>PMVTAATSLRRALENPDSFIVAPGVYDGL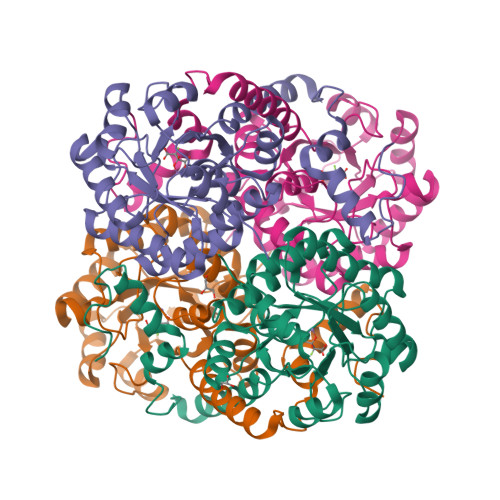SARVALSAGFDALYMTGAGTAASVHGQADLGICTLNDMRANAEMISNISPSTPVIADADTGYGGPIMVARTTEQYSRSGVAAFHIEDQVQTKRCGHLAGKILVDTDTYVTRIRAAVQARQRIGSDIVVIARTDSLQTHGYEESVARLRAARDAGADVGFLEGITSREMARQVIQDLAGWPLLLNMVEHGATPSISAAEAKEMGFRIIIFPFAALGPAVAAMREAMEKLKRDGIPGLDKEMTPQMLFRVCGLDESMKVDAQAGGAAFDGGVDLK[16x]>VQEPLRVPPSAPARLVVLASGTGSLLRSLLDAAVGDYPARVVAVGVDRECRAAEIAAEASVPVFTVRLADHPSRDAWDVAITAATAAHEPDLVVSAGFMRILGPQFLSRFYGRTLNTHPALLPAFPGTHGVADALAYGVKVTGATVHLVDAGTDTGPILAQQPVPVLDGDDEETLHERIKVTERRLLVAAV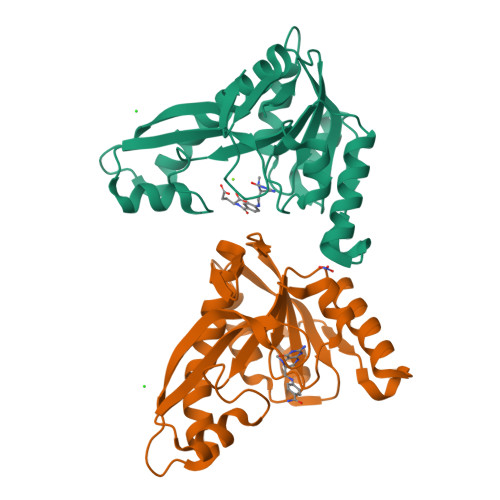AALATHGVTVVGRTATMGRKVTIG[2x]>SNAMNNIRLLNQNDLDSYIELMKFGHHNYEWDRYYLENVSIDRLKTILSNHTDYWNIFGAFEDDEL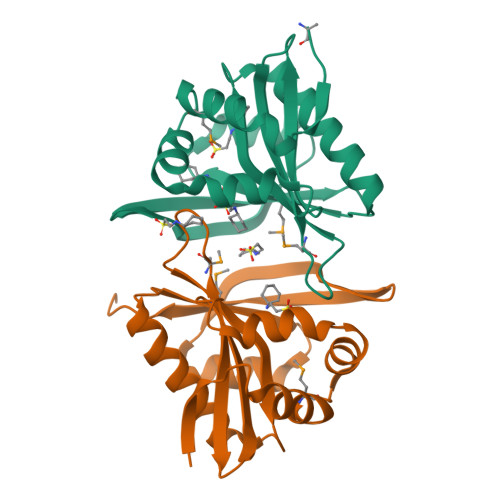VATCTLKQMNYVGKCHKAILENNFVKNNDEIVNRELINHIIQYAKEQNIETLMIAIASNNISAKVFFSSIGFENLAFEKNASKIGNEYFDENWLIYSTTESSD[4x]>[2x]ELICIVQRVNESFSLHSGFGGNVYSMKTEPMTGFTNVTKGASVINQKDWIGFGDARTDLTNDQFPASSDVPLAVAKKFRSLSGASLMLSAFGPPGKVDYLYQGCGKEKVFYEGVNWSPEAGIDCFGSNWTQTKKDFYSRIYEAARSSTCMTLVNSLDTKISSTTATAGTASSCSSSWMKSPLWYAESSVNPGAKPQVCGTEQSATFTLPTSFGIYKCNKHVVQLCYFVYENKAKFNTFGCGDYYQNYYDGNGNLIGGMDNRVAAYRGIANAGVKIECPSKILNPGTYSIKSTPRFLL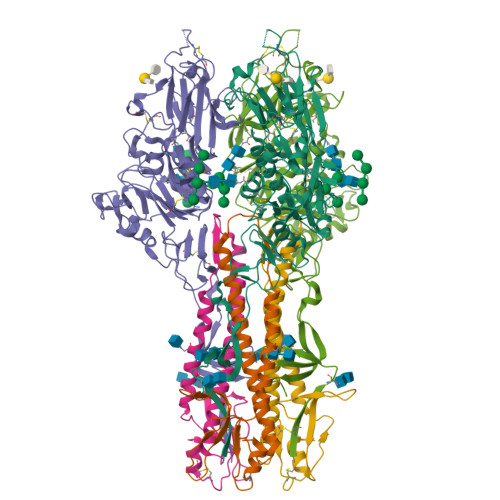VPKRSYCFDTDGGYPIQVVQSEWSASRRSDNATEEACLQTEGCIFIKKTTPYVGEAADNAGDIEMRQLLSGLGNNDTVCVSQSGYTKGETPFVKDYLSPPKYGRCQLKTDSGRIPTLPSGLIIPQAGTDS;>FGLLFVGFVAGGVAGGYFWGRSNGGGGGASVSSTQAGFDKIGKDIQQLRNDTNAAIEGFNGRIAHDEQAIKNLAKEIEDARAEALVGELGIIRSLIVANISMNLKESLYELANQITKRGGGIAQEAGPGCWYVDSENCDASCKEYIFNF[2x]>AEGTRGRSSTARCSLFGSDFVNTFDGSMYSFAGYCSYLLAGGCQKRSFSIIGDFQNGKRVSLSVYLGEFFDIHLFVNGTVTQGDQRVSMPYASKGLYLETEAGYYKLSGEAYGFVARIDGSGNFQVLLSDRYFNKTCGLCGNFNIFAEDDFMTQEGTLTSDPYDFANSWALSSGEQWCERASPPSSSCNISSGEMQKGLWEQCQLLKSTSVFARCHPLVDPEPFVALCEKTLCECAGGLECACPALLEYARTCAQEGMVLYGWTDHSACSPVCPAGMEYRQCVSPCARTCQSLHINEMCQERCVDGCSCPEGQLLDEGLCVESTECPCVHSGKRYPPGTSLSRDCNTCICRNSQWICSNEECPGECLVTGQSHFKSFDNRYFTFSGICQYLLARDCQDHSFSIVIETVQCADDRDAVCTRSVTVRLPGLHNSLVKLKHGAGVAMDGQDVQLPLLKGDLRIQHTVTASVRLSYGEDLQMDWDGRGRLLVKLSPVYAGKTCGLCGNYNGNQGDDFLTPSGLAEPRVEDFGNAWKLHGDCQDLQKQHSDPCALNPRMTRFSEEACAVLTSPTFEACHRAVSPLPYLRNCRYDVCSCSDGRECLCGALASYAAACAGRGVRVAWREPGRCELNCPKGQVYLQCGTPCNLTCRSLSYPDEECNEACLEGCFCPPGLYMDE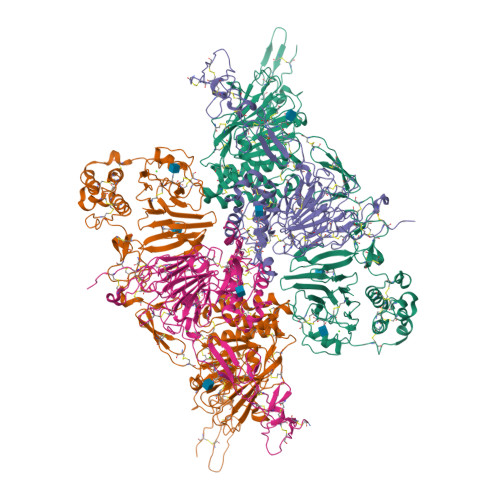RGDCVPKAQCPCYYDGEIFQPEDIFSDHHTMCYCEDGFMHCTMSGVPGSLLPDAVLSSPLSHRSKR[2x];>[2x]SLSCRPPMVKLVCPADNLRAEGLECTKTCQNYDLECMSMGCVSGCLCPPGMVRHENRCVALERCPCFHQGKEYAPGETVKIGCNTCVCQDRKWNCTDHVCDATCSTIGMAHYLTFDGLKYLFPGECQYVLVQDYCGSNPGTFRILVGNKGCSHPSVKCKKRVTILVEGGEIELFDGEVNVKRPMKDETHFEVVESGRYIILLLGKALSVVWDRHLSISVVLKQTYQEKVCGLCGNFDGIQNNDLTSSNLQVEEDPVDFGNSWKVSSQCADTRKVPLDSSPATCHNNIMKQTMVDSSCRILTSDVFQDCNKLVDPEPYLDVCIYDTCSCESIGDCACFCDTIAAYAHVCAQHGKVVTWRTATLCPQSCEERNLRENGYECEWRYNSCAPACQVTCQHPEPLACPVQCVEGCHAHCPPGKILDELLQTCVDPEDCPVCEVAGRRFASGKKVTLNPSDPEHCQICHCDVVNLTCEACQEPGGLVVPPHHHHHH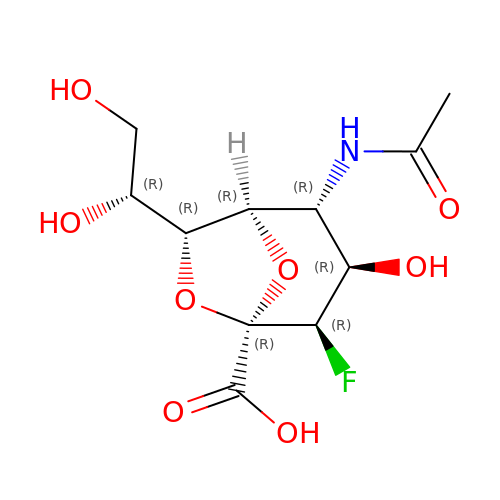(1R,2R,3R,4R,5R,7R)-2-(acetylamino)-7-[(1R)-1,2-dihydroxyethyl]-4-fluoro-3-hydroxy-6,8-dioxabicyclo[3.2.1]octane-5-carboxylic acid | C11 H16 F N O8 | JCWSZUBTEOFKAD-DAXAGCIGSA-N N-(biphenyl-4-ylsulfonyl)-D-leucine 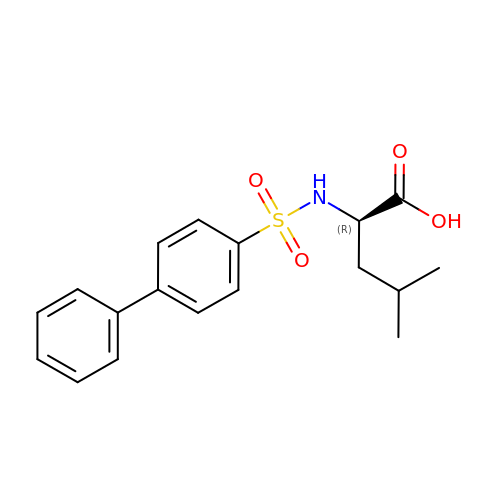| C18 H21 N O4 S | FBSVJQQVDISETN-QGZVFWFLSA-N>[2x]MTRATLLT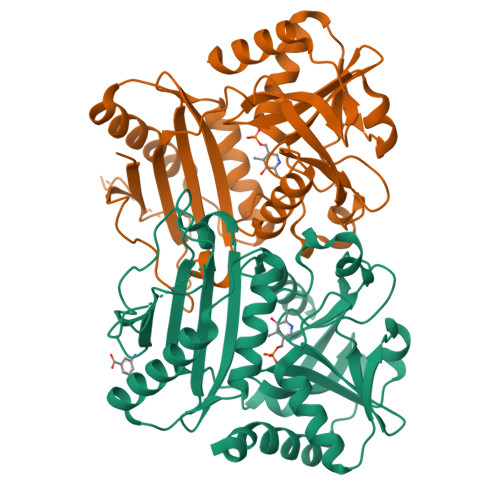VTAPTRPASADEHGADRAAGDAGFVLADFGAPQVRITDLGITRGDGVFETIAVIDGHPQALELHLGRLAHSAALLDLPEPDAAVWREAVLAGVADYRSRNGDGGELFAKLILTRGIEGEGRPSGWVFVDEGEDFSQQRLGIRVVTLDRGYRHDVAETSPWLLAGAKSLSYATNRAAGREAARRGADDVIFVSSDGYALEGPTSNVIVLADGVVRTPQTDQGILAGTTQAAVFDFFEERGYPTEYRRISADELRDAEALWLVSSVRQAAPITALDDREYPVDAALTADLNAYLLARTDLEHHHHHH>MPLLVEGRRVRLPQSAGDLVRAHPPLEERARLLRGQSVQQVGPQGLLYVQQRELAVTSPKDGSISILGSDDATTSHIVVLRHTGNGATCLTHCDGTDTKAEVPLIMNSIKSFSDHAQCGRLEVHLVGGFSDDRQLSQKLTHQLLSEFDRQEDDIHLVTLCVTELNDREENENHFPVIYGIAVNIKTAEIYRASFQDRGPEEQLRAARTLAGGPMISIYDAETEQLRIGPYSWTPFPHVDFWLHQDDKQILENL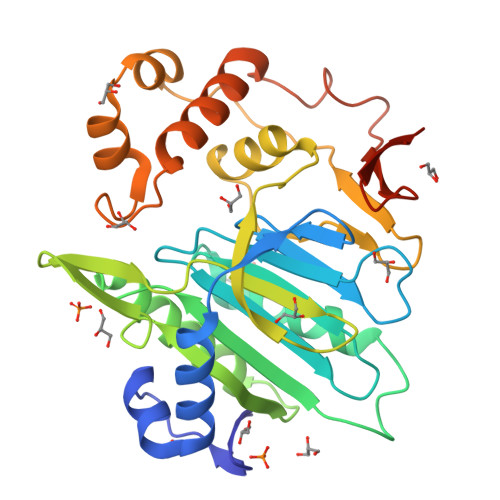STSPLAEPPHFVEHIRSTLMFLKKHPSPAHTLFSGNKALLYKKNEDGLWEKISSPGSLEHHHHHH[2x]>[3x]GPLGSEVKKKKNKKKNKKVNGLPPEIAAVPELAKYWAQRYRLFSRFDDGIKLDREGWFSVTPEKIAEHIAG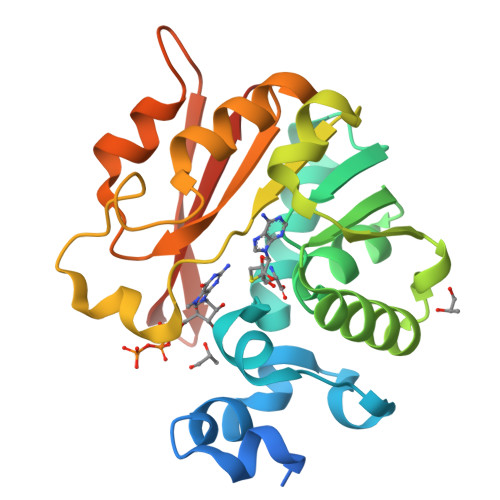RVSQSFKCDVVVDAFCGVGGNTIQFALTGMRVIAIDIDPVKIALARNNAEVYGIADKIEFICGDFLLLASFLKADVVFLSPPWGGPDYATAETFDIRTMMSPDGFEIFRLSKKITNNIVYFLPRNADIDQVASLAGPGGQVEIEQNFLNNKLKTITAYFGDLIRRPASET>GSAQTFEIKGNDLWDPTTFDALRRQLIPSFDLIYEAAVRTVAATVPTAPRVLDLGAGTGLLSAAILRELPDSEVVLVDRSELMLTQARGRFASQDGVTVQTGDLTDPLPEGGFDAVVSGLAIHHLSHTGKRDLFRRIREALRPGGVFVNVEQVQGPLPHLESLYDSQHELHVIREQAPAHEWAAGRERMKFDVCIDLETQLQWLRDAGFRSVDCLAKDFRFATYAGWVS[2x]

Here, we characterize the O-methyltransferases BelI and CysG, which catalyze the initial step of β-lactone formation. Employing techniques such as crystallography, computational analysis, mutagenesis, and activity assays, we identified a His-His-Asp (HHD) motif in the active sites of the two enzymes, which is crucial for binding a catalytically active calcium ion. As expected, BelI as well as CysGΔN16 adopt the class I methyltransferase Rossmann fold, characterized by a core domain of a seven-stranded β-sheet flanked by α-helices. The HHD-motif enables regiospecific C1-carboxy group methylation of their respective malic substrates.

The crystal structures of CysGΔN16 in complex with S-adenosylhomocysteine (SAH) and BelI bound to SAM were solved at 1.5 Å and 1.95 Å, respectively. The 2Fo-Fc electron density maps depict the cofactors at atomic resolution and illustrate similar interactions with protein residues of either BelI or CysG. Intriguingly, the crystal structures of CysGΔN16 and BelI revealed a His122-His123-Asp191 (HHD) motif with additional strong positive electron density, indicative of a divalent metal ion. Molecular analysis indicates that a flexible N-terminus in both enzymes likely plays a key role in substrate binding. Furthermore, phenylalanine in BelI and tyrosine in CysG, at position 18, act as gatekeepers (see below) and can either adopt an open or closed conformation important for catalysis.> SFNIQSDDLLHHFEADSNDTLLSAALRAELVFPYECNSGGCGACKIELLEGEVSNLWPDAPGLAARELRKNRFLACQCKPLSDLKIKVINRAEGRASHPPKRFSTRVVSKRFLSDEMFELRLEAEQKVVFSPGQYFMVDVPELGTRAYSAANPVDGNTLTLIVKAVPNGKVSCALANETIETLQLDGPYGLSVLKTADETQSVFIAGGSGIAPMVSMVNTLIAQGYEKPITVFYGSRLEAELEAAETLFGWKENLKLINVSSSVVGNSESSYPTGYVHEIIPEYMEGLL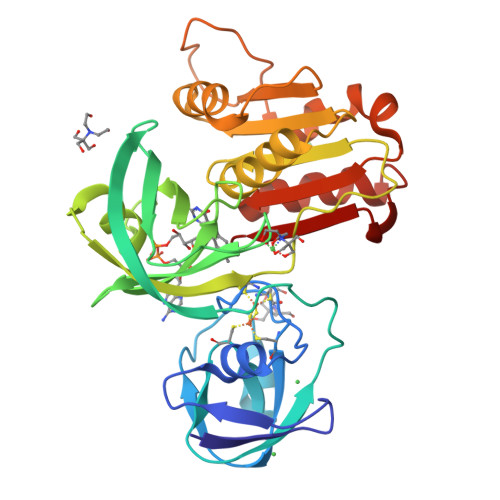GAEFYLCGPPQMINSVQKLLMIENKVPFEAIHFDRFF>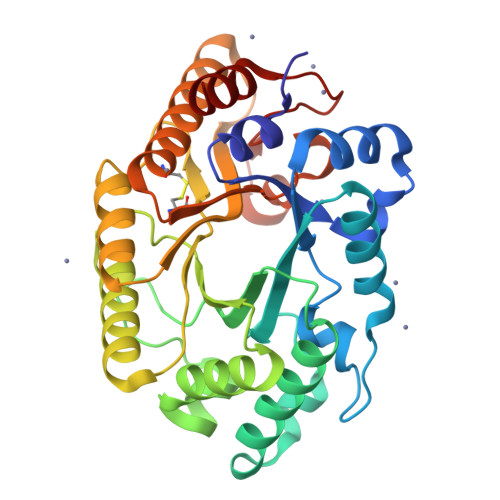 DTATLGELAEAKGRYFGSATDNPELPDTQYTQILGSEFSQITPENTMKWQYTEPSRGRFDYTAAEEIVDLAESNGQSVRGHTLVWHNQLPSWVDDVPAGELLGVMRDHITHEVDHFKGRLIHWDVVNEAFEEDGSRRQSVFQQKIGDSYIAEAFKAARAADPDVKLYYNDYNIEGIGPKSDAVYEMVKSFKAQGIPIDGVGMQAHLIAGQVPASLQENIRRFADLGVDVALTELDIRMTLPRTAAKDAQQATDYGAVVEACLVVSRCVGITVWDYTDKYSWVPSVFPGQGAALPWDEDFAKKPAYHAIAAALN> MMLLTRHA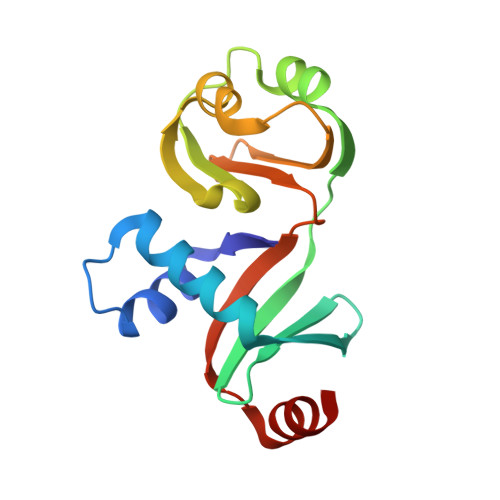KERIAKRLAKKRSLSHIYSSLWAFLERAVRIEIAEGVVAFTDGRKTLVCVPLDCERLSRGEILEKVRGVGVYECIFPEGRLAKLTRPEKFLESVPPGEYYFYMNDEKKVLYVGKRRPLLAITFRPAKRDERLFYIWA yatakemycin-adenine nucleobase adduct | C40 H34 N10 O8 S | 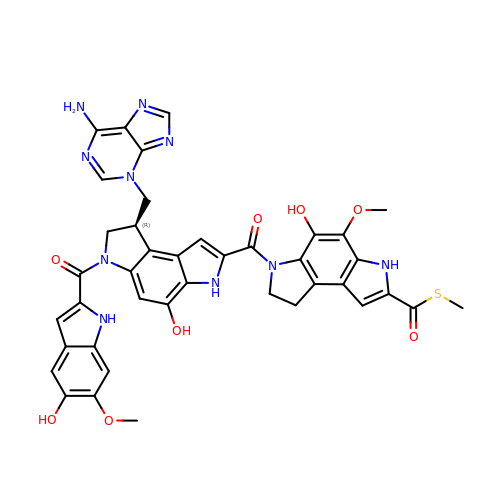FJMCEQLVMJYVHU-QGZVFWFLSA-N>[3x]SMVKIYAPASIGNVSVGFDVLGAAVSPIDGTLLGDCVSVTAAERFSLHNEGRFVSKLPDDPKQNI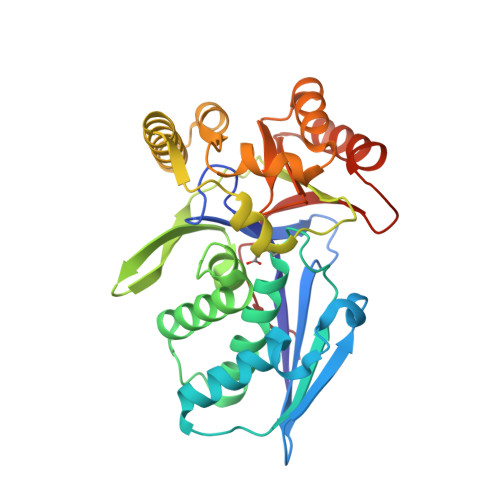VYQCWERFCQEMGKEIPVAMVLEKNMPIGSGLGSSACSVVAGLMAMNEFCGQPLDKVTLLGMMGELEGRVSGSIHFDNVAPCYLGGMQLILEQEGYISQDVPGFSDWLWVMAYPGIKVSTAEARAILPAQYRRQDCITHGRNLAGFIHACHTQQPDLAAKMMKDVIAEPYRTQLLPGFAAARQAAQDIGALACGISGSGPTLFAVCNDQATAQRMAGWLQNHYLQNDEGFVHICRLDTAGARLLG>[2x]GPLGSDYIIKEKTVLLQKKDSEGFGFVLRGAKAQTPIEEFTPTPAF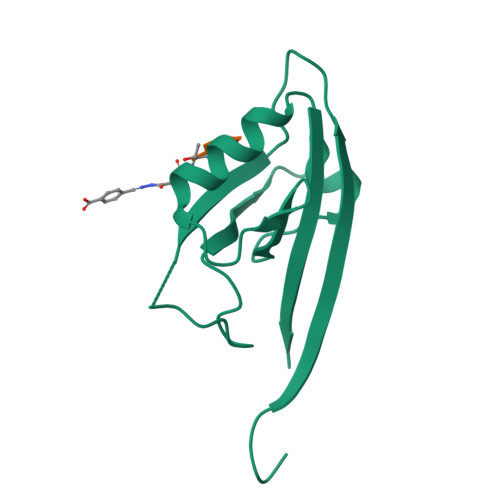PALQYLESVDEGGVAWRAGLRMGDFLIEVNGQNVVKVGHRQVVNMIRQGGNTLMVKVVMVTRHPDM;>TRL[2x]>MAHHHHHHMSTMMIFTGNANPELALKISSHLQIPIGKATVGTFSDGETMVEILENVRGKDVFVLQSTCAPANNNLMELLIMADALRRSSAGRITAVVPYFGYARQDRRVRSARVPITAKVVADMMASVGICRVLTVDLHADQIQGFFYMPVDNVYSTPVLLEDITKQKLNNIMIVSPDVGGVVRARAVAKRLNDAELSIIDKRRSGPNKSEVMHIIGEPANKNCIIVDDIVDTAGTLCTAAHELKKNGAKSVRAYITHPVLSGPAVNNIKHSGLDEVVVTDTIPLSAEAQNCEKIRVVSLADMLAQAIKRVNV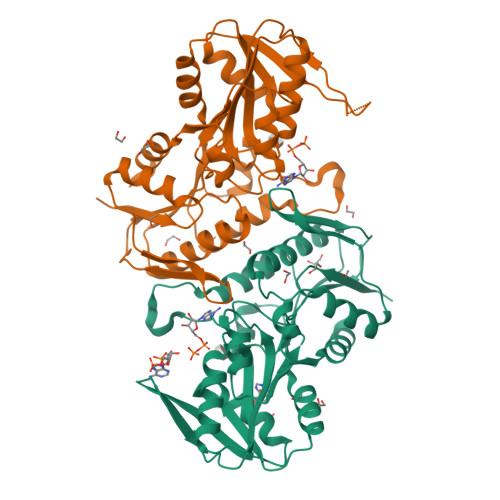EESVSSMFAE[2x]5-{3-[3-(1,3-benzodioxol-5-yl)-5-methoxyphenyl]prop-1-yn-1-yl}-6-ethylpyrimidine-2,4-diamine 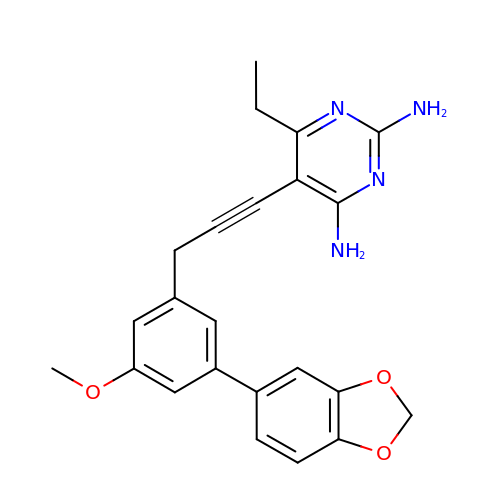| C23 H22 N4 O3 | DEWBMLVREOXAJX-UHFFFAOYSA-N>[2x]DEPQLLHGAGICKWFNVRMGFGFLSMTARAGVALDPPVDVFVHQSKLHMEGFRSLKEGEAVEFTFKKSAKGLESIRVTGPGGVFCIGSERRPKGGDRCYNCGG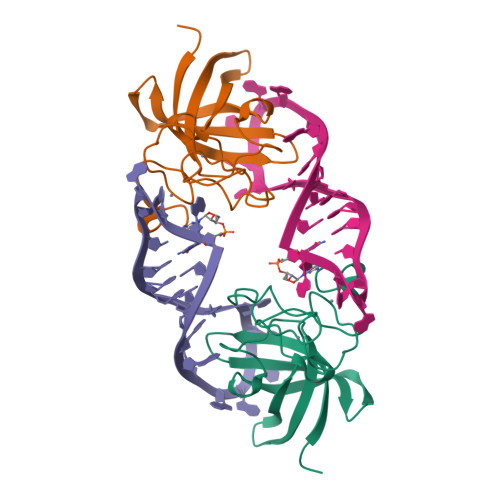LDHHAKECKLPPQPKKCHFCQSINHMVASCPLKAQQGPSSQGK>TRDQNGTWEMESNENFEGYMKALDIDFATRKIAVRLTQTKVIDQDGDNFKTKTTSTFRNYDVDFTVGVEFDEYTKSLDNRHVKALVTWEGDVLVCVQKGEKENRGW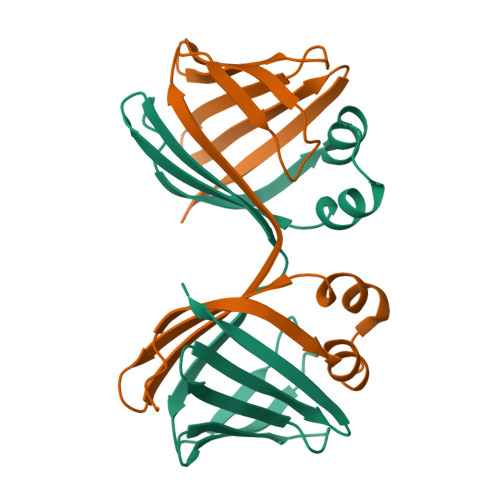KQWIEGDKLYLELTCGDQVCRQVFKKK[12x]> DGDQSET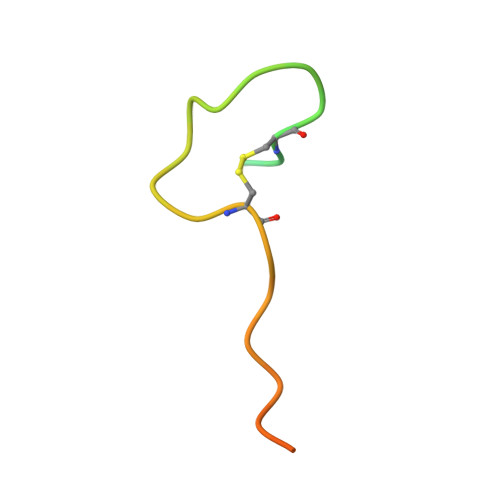SPSQNQGKCKNGLGEYTCTSLEGFEGKNSELF> AEAEFGCPDNGMSEEARQKFLEMHNSLRSSVALGQAKDGAGGNAPKAAKMKTMAYDCEVEKTAMNNA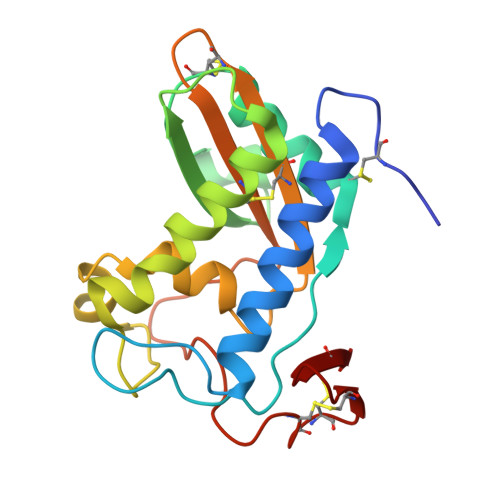KQCVFKHSQPNQRKGLGENIFMSSDSGMDKAKAAEQASKAWFGELAEKGVGQNLKLTGGLFSRGVGHYTQMVWQETVKLGCYVEACSNMCYVVCQYGPAGNMMGKDIYEKGEPCSKCENCDKEKGLCSA The rational design of small molecules that target specific DNA sequences is a promising strategy to modulate gene expression. This report focuses on a diamidinobenzimidazole compound, whose selective binding to the minor groove of AT DNA sequences holds broad significance in the molecular recognition of AT-rich human promoter sequences. The specialized method of X-ray crystallography was utilized to investigate how the sequence-dependent recognition properties in general, A-tract, and alternating AT sequences affect the binding of diamidinobenzimidazole in the DNA minor groove. A strong and direct hydrogen bond between the N-H of the benzimidazole and an H-bond acceptor atom in the minor groove is essential for DNA recognition in all sequences described. In addition, the diamidine compound specifically utilizes an interfacial water molecule for its DNA binding.

Likewise, for A6-DB1476, we also presented a structure with two possible ligand orientations. The A6-DB1476 complex is reported at a resolution of 2.1 Å. The electron density map showed no clear preference for one DB1476 orientation. Therefore, the ligand was refined in two orientations within the ligand’s electron density map, and both orientations fit the density somewhat similarly. The final statistics show that A6-DB1476-I and A6-DB1476-II have slightly different Rfree values, 31.0 and 32.5%, respectively, and different average B-factor values, 48.8 and 45.1, respectively. However, in both A6-DB1476 structures, the two amidines in each of both DB1476 orientations participate in an H-bond interaction with only strand B. The DB1476 preference for one strand is not completely understood since the compound can readily form strong hydrogen bond with the available N3 of adenine in the minor groove. Therefore, as much as DB1476 may have a preferential binding orientation across the minor groove, the structure of A6-DB1476 suggests that DB1476 can still adopt differential binding configurations in the minor groove of different AT DNA sequences to account for unfavorable interactions. A6-DB1476 has a higher DNA twist in the minor groove, suggesting an overall increase in rigidity.

> CGCAAAAAAGCG;> CGCTTTTTTGCG> MLDPNLLRNEPDAV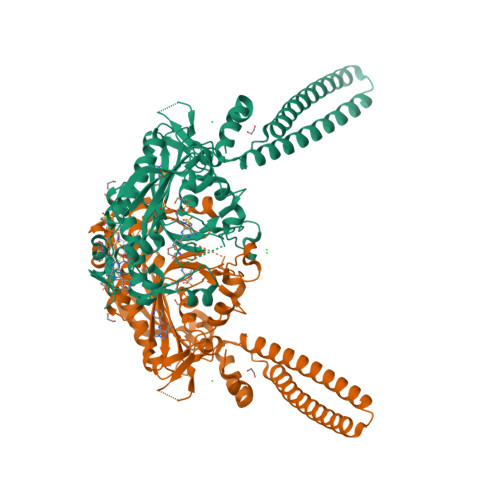AEKLARRGFKLDVDKLGALEERRKVLQVKTENLQAERNSRSKSIGQAKARGEDIEPLRLEVNKLGEELDAAKAELDALQAEIRDIALTIPNLPADEVPVGKDENDNVEVSRWGTPREFDFEVRDHVTLGEMHSGLDFAAAVKLTGSRFVVMKGQIARMHRALSQFMLDLHTEQHGYSENYVPYLVNQDTLYGTGQLPKFAGDLFHTRPLEEEADTSNYALIPTAEVPLTNLVRGEIIDEDDLPIKMTAHTPCFRSEAGSYGRDTRGLIRMHQFDKVEMVQIVRPEDSMAALEEMTGHAEKVLQLLGLPYRKIILCTGDMGFGACKTYDLEVWIPAQNTYREISSCSNVWDFQARRMQARCRSKSDKKTRLVHTLNGSGLAVGRTLVAVMENYQQADGRIEVPEVLRPYMNGLEYIGELALVPR>GKAFDDGAFTGIREINLSYNKETAIGDFQVVYDLNGSPYVGQNHVSFITGFTPVKISLDFPSEYIMEVSGYTGNVSGYVVVRSLTFKTNKKTYGPYGVTSGTPFNLPIENG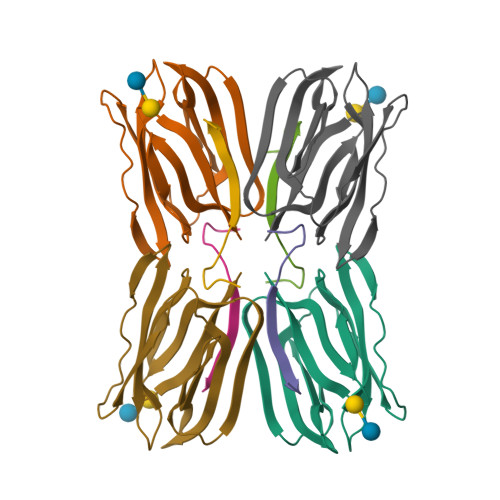LIVGFKGSIGYWLDYFSMYLSL[2x];>[4x]DEQSGISQTVIVGPWGAKSS;>GKAFDDGAFTGIREINLSYNKETAIGDFQVVYDLNGSPYVGQNHKSFITGFTPVKISLDFPSEYIMEVSGYTGNVSGYVVVRSLTFKTNKKTYGPYGVTSGTPFNLPIENGLIVGFKGSIGYWLDYFSMYLSL[2x]> GLPVLNTPGSNQYLTSDNYQSPC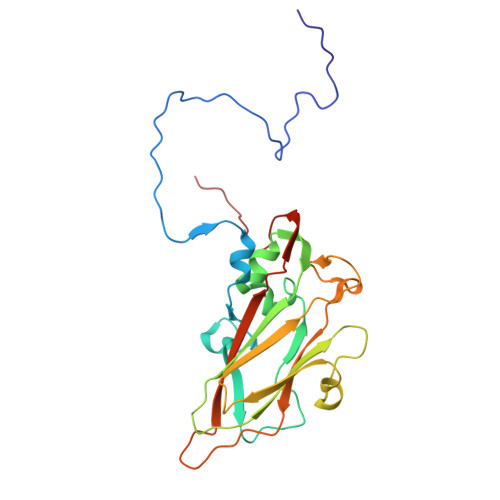AIPEFDVTPPIDIPGEVKNMMELAEIDTMIPLNLENTKRNTMDMYRVTLSDSADLSQPILCFSLSPASDPRLSHTMLGEVLNYYTHWAGSLKFTFLFCGSMMATGKILVAYAPPGAQPPTSRKEAMLGTHVIWDLGLQSSCTMVVPWISNVTYRQTTQDSFTEGGYISMFYQTRIVVPLSTPKSMSMLGFVSACNDFSVRLLRDTTHISQSALPQ> WTVAVYCAASPTHAELLELAA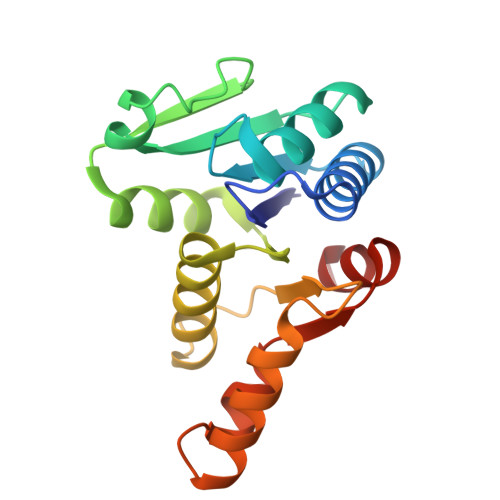EVGAAIAGRGWTLVWGGGHVSAMGAVASAARACGGWTVGVIPKMLVYRELADHDADELIVTDTMWERKQIMEDRSDAFIVLPGGVGTLDELFDAWTDGYLGTHDKPIVMVDPWGHFDGLRAWLNGLLDTGYVSPTAMERLVVVDNVKDALRACAPS>[2x]MINQNATYMEESAQSAVDNFGLGFNLGNTLDANGCGTGKPVATYETFWGQPETTQDMMTFLMQNGFNAVRIPVTW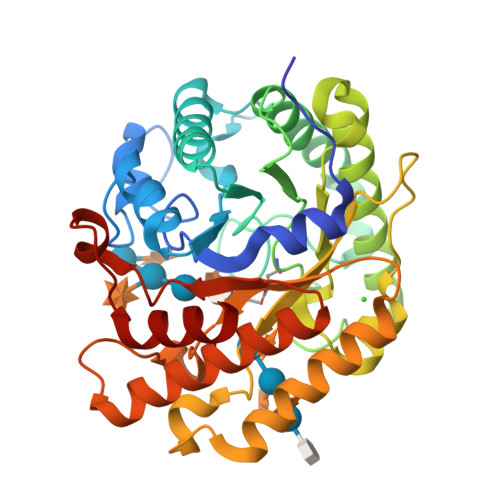YEHMDAEGNVDEAWMMRVKAIVEYAMNAGLYAIVNVHHDTAAGSGAWIKADTDVYAATKEKFKKLWTQIANALADYDQHLLFEGYNEMLDGNNSWDEPQKASGYEALNNYAQDFVDAVRATGGNNATRNLIVNTYAAAKGENVLNNFMLPTDAVNNHLIVQVHSYDPWNFFNTKTTWDSECHNTLTEIFSALSKKFTTIPYIIGEYGTHGESDISVSKSSPAEKIKLAADQAADMVKLAKDHHSATFYWMSIFDGSDRIQPQWSLPTVVEAMQEAYNN> MAENYGLTGSGFNLPPMDDLVQETKKTFKSAFGEDFNTESNSVADKLIQIFNEREYQLWLLMGSVYYAQTMQGAEGIY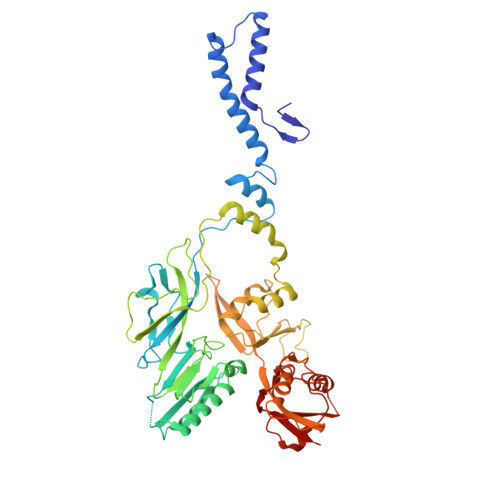LDDLLGKRGIYRLGKTRSTGTVVMTIDSSVPYNMIYSAATYTIDTDYELSSDVQVAGNIVAQLIKGTDLSVGTYRLQIQNTTDQSVKTLSLNLTATSGQPLITFFGQIKDFIVNNTILSNQDRIWIDSTEGALYIGYDTNKIMIGLSSRVDFRTNPMAGTRSISMDVRSIEPGYISRDVHSVRSINPTPGGFVDIDNLSAFIDGSDVESDNEYRIRAATSISEGKATRPAILAALLNKVEGIEKVRIFNNNTDKTNSLGIPPYRFMVVCYGGGTAEISQVLYDTIATSNNTYGDTFYDITTEDDQVERIWHTKAAARQLAIRVRYRGRPLSLTEETAIANGLATAVNGTMIAGTLYNVRLVGTVMSSTSPDRFTQVYVDIKNKGQPDSAYVNTDVTASTTQVLSLELEDVIFSQIV The phylum of Apicomplexa groups intracellular parasites that employ substrate-dependent gliding motility to invade host cells, egress from the infected cells, and cross biological barriers. The glideosome-associated connector (GAC) protein is a central bridging component of the gliding machinery. This large protein composed of numerous armadillo repeats (ARMs) is highly conserved throughout the Apicomplexa phylum and links F-actin to the TRAP/MIC family of surface adhesins at the plasma membrane, which targets host cell ligands and mediates adherent anchor points. GAC facilitates the association of actin filaments with surface transmembrane adhesins and the efficient transmission of the force generated by myosin translocation of actin to the cell surface substrate.

Well-diffracting and reproducible crystals were obtained at pH 5 for native full-length TgGAC (residues 1–2639; Kumar et al., 2022). The structure was solved by multiple-wavelength anomalous dispersion (MAD) to 2.7 Å resolution with an Rfree of 26%. The electron density for residues 7–2504 was of sufficient quality to facilitate modelling for these residues. The remaining electron density showed evidence of peptide backbone but could not be confidently modelled and refined, indicating a degree of conformational flexibility for residues 2505–2639. The crystal structure of TgGAC7–2504 comprises 169 helices arranged in 53 consecutive helical bundles that resemble ARM and HEAT-like repeats (AHRs; Kippert and Gerloff, 2009) linked to the mixed α/β C-terminal PH domain. RI (residues 1–1665) comprises 37 consecutive AHRs of approximately 40 residues long that are supercoiled into a three-layer pyramid structure. RII comprises 16 canonical armadillo repeats (AHR38-53) and forms a superhelical arch that contacts the base of the RI pyramid helical regions. This interface encompasses a surface area of 1550 Å2, with AHR1 and AHR17-18 from RI forming one side while AHR48-50 from RII form the other. The interface comprises several prominent electrostatic interactions (K2254-D11, E2436-H24, D2330-R629, D2346-K672, and D2197-R716). Remarkably, the overall architecture of the predicted structures is very similar to that observed in the crystal structure of TgGAC, as it is characterised by a series of tandem AHRs that are supercoiled into a large ring and is closed by specific interactions between N- and C-terminal AHRs.

> KRNPDAGVATAVQSVIQHQTFKRMLLFGLRSLADFCSPSNQLYQENALDALDRGVLSAIQTAVTTFSDDDDLMLCASRVLWAMSVAIKEEMDPAHIARVHSEGSPVIVAVVNSSPTDPQTIEDSMNFVDNLKRAGAPVDGASLAGGMLSIFTKTALDMKTAKRVTAALAIAAETAEGSTALYNAGGTSVLLTYCLDQGDLSDAGVEMVEGAFDTVRYMAGYQCTDATTLPQCIALMDKYRGRKSASAKGSSALAAMIGPEQLQKCLNTLKTAEAGSAEYDEALVTLGSMSYISSFTDEIVRAGGVPLLIELINSGLPQMEGNPEKIASMISGAAKMLARIASNPVNVDAIVQAGGVATLCTAVSYCTESMEALGALCMALVPLASRESLAHEIVQYQTFATVLPILYQNVESPEIAALAMELVATGSQHEEIQEHMLQNQAAEICSLCCQYHTADASYQQHAISALNRLVPRLTTLHGVSEYGGIQGVIASLNANVNNEQVALLAVQLLDNFSEVSDAKTYMSDGTCVDAVLAAMLEHEGNDLLISAGVHCLARIATEDDCARHLNVLDTAIQTARGNPDGVYRVLAAISGLSRVPSLRQIFEEKNASDTILAGISSWIECSRFEGQNRIIKAALKTVKNMKISGDGDLTSCFAAMCDVACLPQVKRVVELEEPDNNILVADTAAFRDLAATMRITGAENLERCIESVLRVMRKYPDSRRAQLNCLETLNYLAQCDGGEGVAILSRTGGLNAVVQYLTRAPMYLDAQIAGFTVLATSAKIDSNVGETLRKCNCLQALKVAMRTHAKSKELKRTIAPLVALLMPTDALETEIQELLNECASACEKNNFPHLHENLAALNELLISSEGAKIAARLGIGAHMCKYQEYISAHEQDALAVTDYDILGKDLFDATVSECAHAMEQVASTRSGRNALIKAGNVATLISLYESLKAPQSQYSEEAAIHCLEALRILLKSDKRSAELAFERNFVSTLCVGIDSFPHSAPVLGATCACLAAMATTPERVQMLTAQPAFESLLQKLVFVIQNDPSKDNKLVAMRALQELVEITNDATMANKIAEAGAVTALFRIIDEYGDDEQLTVQAAEVLALLGAFEDLRRFYDNDVRFPAQVLTAALTKQKNNETAVVHLLDVLNKLATSEDRAVLRELGVMEQVADAMRVHSESEAVTRLGGELFAKMGADEQIKSLMLQIIETVESGAEDTAQTVDILCGRLAVFLAAPLEDPRDALQHTEKCLGSLVATLQTYPGSERLEGNVALVCRRLCDRCFDDADDPYGAWAVAASGMLAQFAGMVAGETVLANKKFLGPAYRTFTACCANAYCMPTMVEVAPSFLPQTYTLLEMHKNDAETVARVLEFLRYFAEDPTACGLIVQNMSGSSGDVVALTVLLMQQHQNNDAVVCAGMEFLGALAYTLSQAGYEPLPTLADGSVLRDCDALMGSNSSSARQLAHMHMIEKMLLSKAYNDALIQEQALKKLTMSLKAEDDKKRFSDEERAGLYAAMACVLLAAGGAGLTGEMEKFNGFEVVLQAIEEFGENPTVIKEVNRALQGLSMADVNMTARTVKEAVPKLCTEATTAIQTDAECADTFCDLMLQLVSQEGNGRQLLQVYGLEETLQGVENLAAYYGEDFGTQLSEKVAMIRQAMEDDQPREKTCKDVYDLLNSRVQQGLSVAISEVAILQEEVEFLVSQMGMYNQEQLDHQTAMGADHQYGNMAFELLAATSANVKLLQANEFSKMELALIKGQADPEIVLYAVKALTAFCKFPPAAQDTARIQGCPALVTEACSKINKSGLPNERKEEHLCARYFLVERTAINRNLYNKTPIMTELINSWNDYDKGAYTTTLLRFVFRAMRRVVSDAHVEELLKANVLQRLIGIISDVNADMALLPDVLFLLGSLAVVPEIKTKIGELNGIAACTDLLQRALPKPNTAPVVTNVCLAFANICIGHKKNTEIFSKLGGPALNVKVLNDRGHEYDVCNAASVLLCNLLYKNESMKKLLGTNGAPAALVKGLSNYDGSEEKTAIRCLESVFKAISNLSLYTPNIQPFLDAGIENAYSTWLSNLSETFPDAQLETGCRTLVNLVMENEENNMRKFGVCLLPCMAVAKQGRTDTKALLLLLDIEASLCRLKENAEAFAANGGIETTIRLIHQFDYDVGLLTLGIHLLGIQSAVKDSIQRMMDADVFSILVGCVEVDAEGNEVTDLVVGGLRCTRRIVRSEELAFEYCNAGGIATIANVICKSINQPMVMLEACRVLLGLLFYTTRSQADRQAAVEALHAQCQQRAEQMHAQAQADYEAGVVSEPPPEEMEVPEPDPDELANAAYGGWYQMGMDEVMIDAILQAVCACAAVEAHAKQLRLQRVCLGLAAYFASEQMGTSSLVGSGIEQVLTQIMTNFAGEGTTMQLSCVIINSIAMTSGDMYEEIKTSALLSALKTSVGKMATKKPEEKALKETCAATLEAASSGEDPFDAFSKTVTELDFKFTEWNVDPYP> MKDNSTSAVSSWLGYKIQEYRLTQRLLEANNSSCIGFEILDDLEEHTGSTSTFEQDKISTTGRNIVSNHSKDLWKTLSNWMDLIDSGEIDVDNTIFLLFTNKRCHSEVLQLLSTSQATEEASKAFDEILKIVSHPSPSIANYLNNFSKSKTDACRLISKFTYIYGSGSAPHDLRESYKLHRLGALEEHLDEIMYEILGWVSDVLTLAAEKRQPTIVRAKDFGARLGEIESKYRQKTILNYFCNRSSESEDVQNTIKDAPNYIKQLNLINVDDSELEEAAIANLETKDAVVEWTLNGDVQDYSYRYYQRELRRCWGIQKQKIHLDFNGRPETEVGQRLYIECLNNVTRYYLENKKVGDFFAHGTLHSMADKLTIGWHPEFDKKLGDPDA;>[2x]MFFQIEKVVLWSKEAKHKPRVIEFALNKVNLITGSSKSGKSSLIPIIDYCLGSSKCSIPVNTIRDTTAWYGVQIKTKHSRLLIARRDPSNQLSTSNAFFVEAENIEIPQNIEKHNVNIDTVKNRLNEISGVSNISFDFYDTGRIDKKRTSTRDLSAFNYQPQNIIANPNALFYKTDSFEHKSKLVTILPYVLGALSNTDIENQHRIKNLEEEYRKVERRLLKLKRQNEDWLSSAQAYVIKAMELGLVNSDKDIYQLKPERLLNVLKNIATKEIDYSTSAANIKYASEQEAEITKRSRDISNNLAKVKSRLQNINSMNRLANTHSDASRLKRERLSLSKWLLTQNDINSSLFSEPNEIRSLVLEPLARAFSNLEAELEVPIHVQGALSREKIYLEGELTRLASEMKDVNTQLKILRGNKRKLGYDAFSVGKFVGEVEKALSLMGESESESELSKEYKRLKKELSVLRLKIDPREFERK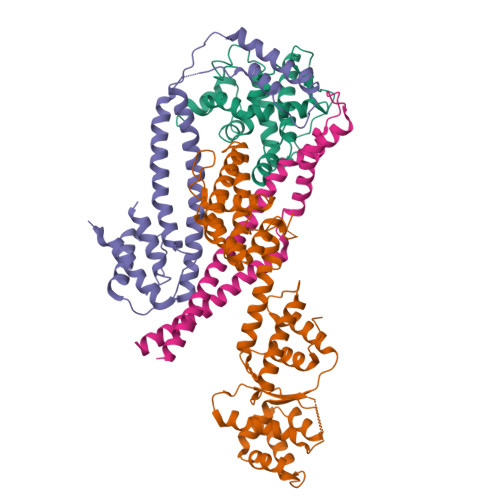TKLQLAKVNKLASDWLPHLDTENPNAPISLHEKELTITVNSSGREDYLWEIGSGANWLSYHVAITLALHQHFSSLEASPVPNYIIYDQPSQVYFPSKLRHQATPEEDELALLEQDEDIVQVKKIFEAFNGAIEKTKDNLQIIVLDHAPSTLVKSIPKGHLVEEWRNGIKLIPLDWL;> MIKNLEIQMLKPENNLEKEAWEINNPAMCSYMLWIATLAYYQKQKEPIHPSRLFCLFPFILYSDTRNVLLSSKGSLKSYLAKFSNSKAISGDIPLSIHFRIDIQKNKTLDALIVAFDSGLLVIDSDSGLIKPNVSIKPLPNSKLTDTIKELVYCSTKIGRWLSEMTNQDLARDLKVIF>[2x]DELYRQSLEIISRYLREQATGAKDTKPMGRSGATSRKALETLRRVGDGVQRNHETAFQGMLRKLDIKNEDDVKSLSRVMIHV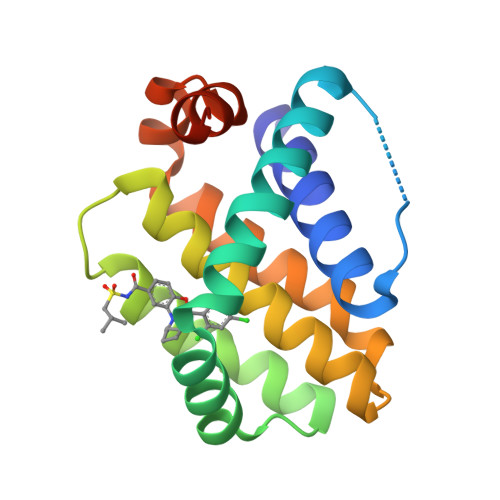FSDGVTNWGRIVTLISFGAFVAKHLKTINQESCIEPLAESITDVLVRTKRDWLVKQRGWDGFVEFFHVEDLEGG> IVGGQECKDGECPWQALLINEENEGFCGGTILSEFYILTAAHCLYQAKRFKVRVGDRNTEQEEGGEAVHEVEVVIKHNRFTKETYDFDIAVLRLK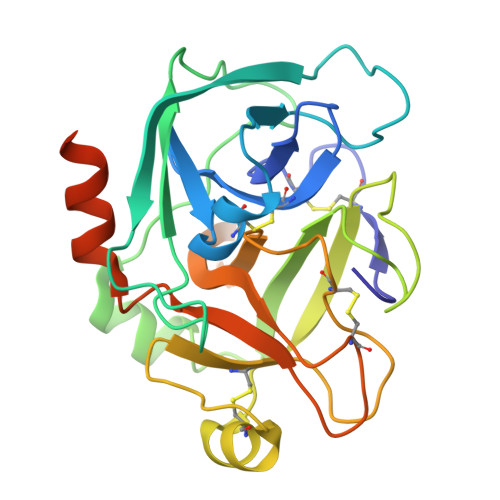TPITFRMNVAPACLPERDWAESTLMTQKTGIVSGFGRTHEKGRQSTRLKMLEVPYVDRNSCKLSSSFIITQNMFCAGYDTKQEDACQGDSGGPHVTRFKDTYFVTGIVSWGEGCARKGKYGIYTKVTAFLKWIDRSMKTRGLPKAKSHAPEVITSSPLK> SPNVEACGYSDRVQQITLGNSTITTQEAANAVVCYAEWPEY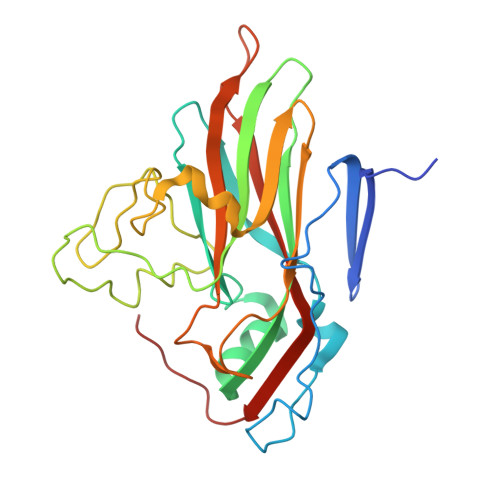LPDVDASDVNKTSKPDTSVCRFYTLDSKTWTTGSKGWCWKLPDALKDMGVFGQNMFFHSLGRSGYTVHVQCNATKFHSGCLLVVVIPEHQLASHEGGNVSVKYTFTHPGERGIDLSSANEVGGPVKDVLYNMNGTLLGNLLIFPHQFINLRTNNTATIVIPYINSVPIDSMTRHNNVSLMVIPIAPLTVPTGATPSLPITVTIAPMCTEFSGIRSKSIVPQ> GPLSMSCWLREQTLLLAEDYISFCSGIQQTPPSESAEAMRYLAKEMEQQHRTKFRSLSQEFLDTCGADPSKCLQSVMRELVGDGKMNWGRVVSIFTFTGVLASELLSRGENSEGSRRLAETIADYLGGEKQDWLVENGGWEGFCRFFHNARQ;> ALWAAKKYGQQLRRMSDEFDKGQMKR

NRZ is a 19 kDa protein expressed in the epiboly of the extra-maternal yolk syncytial layer (YSL) of zebrafish eggs. In vivo, NRZ has been shown to be a potent inhibitor of apoptosis after serum withdrawal, and controls development during somatogenesis and gastrulation. Similar to other pro-survival Bcl-2 proteins, NRZ adopts a conserved Bcl-2-like fold consisting of eight α-helices that form a globular helical bundle. Our findings suggest that NRZ is a unique pro-survival Bcl-2 protein with an unusual pro-apoptotic Bcl-2 binding profile unlike its counterparts in mammalian systems.

NRZ utilizes the canonical hydrophobic binding groove that is also found in other pro-survival Bcl-2 proteins to accommodate the zBad BH3-motif using a combination of hydrophobic and ionic interactions as well as hydrogen bonds. To accommodate the zBad BH3-peptide NRZ undergoes localized conformational changes. Upon binding of the BH3-motif, the C-terminal end of α4-helix moves by 3.0 Å relative to apo-NRZ, thus enlarging the binding groove to accommodate the Bad BH3 motif. Detailed inspection of the NRZ: zBad BH3 complex interface reveals five salt bridges between Lys93Bad and Glu75NRZ, Lys94Bad and Glu56NRZ, Glu105Bad and His46NRZ, Arg100Bad with Asp79NRZ and Asp104Bad with Arg86NRZ. In addition to ionic interactions, the NRZ: zBad interface also features three hydrogen bonds between Arg100Bad–Leu76NRZ, Arg100Bad–Glu75NRZ, Gln98Bad–Lys49NRZ. Finally, the four highly conserved hydrophobic residues Y95, 99L, M102 and F106 from the zBad BH3 motif protrude into the ligand binding groove of NRZ and are accommodated in four hydrophobic pockets at the floor of the binding groove. To validate the structure of NRZ: Bad BH3 we mutated two key NRZ residues involved in ionic interactions, Asp79 and Arg86 to Ala, and examined the ability of these mutants to bind BH3-motif peptides. Both mutants showed substantially reduced binding to Bad, with D79A displaying a tenfold reduction in Bad binding, whereas NRZ R86A displayed a 14-fold reduction in affinity. The binding of zBad to NRZ buries a total of 2366 Å2 solvent accessible surface and solvation energy of isolated structure −10.1 kcal/mol and ΔG of interface formation and dissociation of −3.9 kcal/mol. In contrast, NRZ maintains the ordered α3 helix on binding Bad, which leads to the C-terminal end of α4 helix moving by 3 Å relative to that in apo-NRZ.> ELGDSLEEFLAKATTDKNLARLLVCMGEALRTIAFKVRTASCGATACVNTFGDEQLAVDMLADKLLFEALRHSHVCKYACSEEEPILQDMEGEGFSVAFDPLDGSSIVDTNFTVGTIFGVWPGDKLTGITGRDQAASA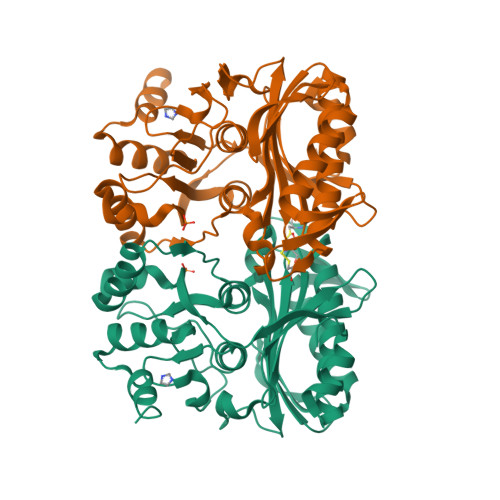MGIYGPRTTYVVAINGFPGTHEFLLMDDGKWQHVKETTEIKEGKLFSPGNLRATFDNADYEKLINYYVSEKYTLRYTGGMVPDVNQIIVKERGIFTNVTSPTTKAKLRLLFEVAPLGLLIENAGGYSSDGKQSVLDKVVVNTDDRTQVAYGSRDEIIRFEETLYGDSRLKAELAAATV;> ELGDSLEEFLAKATTDKNLARLLVCMGEALRTIAFKVRTASCGATACTNTFGDEQLAVDMLADKLLFEALRHSHVCKYACSEEEPILQDMEGEGFSVAFDPLDGSSIVDTNFTVGTIFGVWPGDKLTGITGRDQAASAMGIYGPRTTYVVAINGFPGTHEFLLMDDGKWQHVKETTEIKEGKLFSPGNLRATFDNADYEKLINYYVSEKYTLRYTGGMVPDVNQIIVKERGIFTNVTSPTTKAKLRLLFEVAPLGLLIENAGGYSSDGKQSVLDKVVVNTDDRTQVAYGSRDEIIRFEETLYGDSRLKAELAATVV{2-chloro-5-[({2-[3-(prop-1-en-2-yl)phenyl]propan-2-yl}carbamoyl)amino]phenoxy}acetic 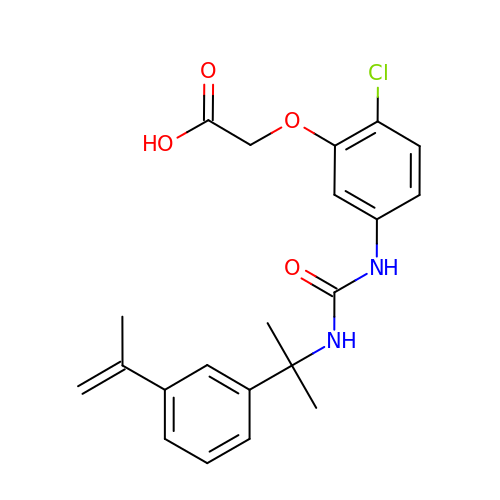acid | C21 H23 Cl N2 O4 | NIAYZIDQFFFUTN-UHFFFAOYSA-N>GPGSEFRQDKMREEGLQLVSMIREGEAAGACPEEIFSALQYSGTEVPLQWLRSELPYVLEMVAELAGQQDPGLGAFSCQEARRAWLDRHGNLDEAVEECVRTRRRKVQELQSLGFGPEEGSLQALFQHGGDVSRALTELQRQRLEPFRQRLWDSGPEPTPSWDGPD[2x];>[2x]DPAMQRCFSA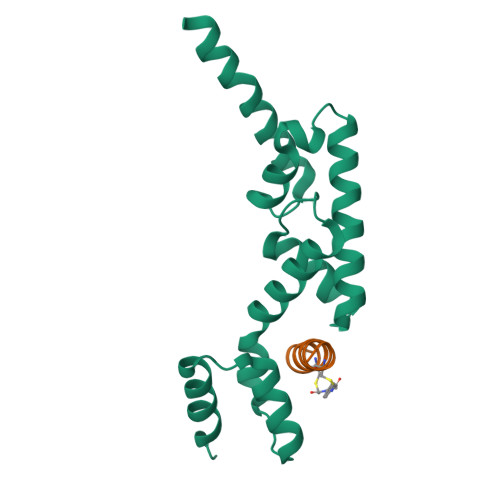AVYCAIS Carbohydrate component from a pentavalent N-acetylneuraminic acid conjugate | C15 H27 N O9 | 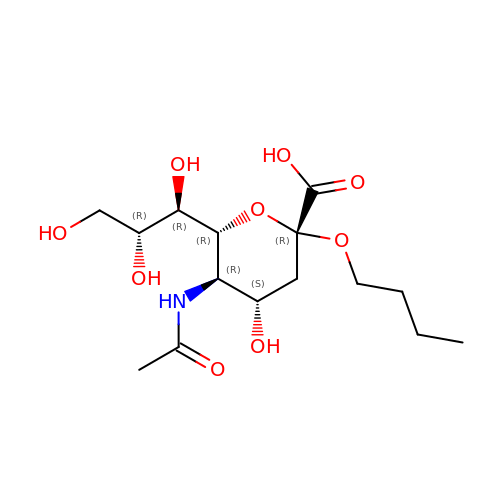HDYHZAZYSDVKLZ-FSTWUICMSA-N(7S)-2-(4-phenoxyphenyl)-7-(1-propanoylpiperidin-4-yl)-4,5,6,7-tetrahydropyrazolo[1,5-a]pyrimidine-3-carboxamide | C27 H31 N5 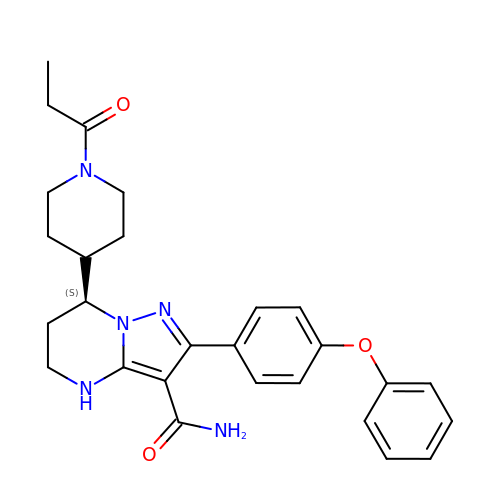O3 | WVLVCHIIZKJCHR-QFIPXVFZSA-N>[4x]HHHHHHSSGLVPRGSHMLRRTSSTFSAKRVFVVGGHITTFVGKGSPLFIDKKHPDFGKKENKTLEELLAESINGALQNTGLHDGRAALVDKLVVGNFLGELFSSQGHLGPAAVGSLSGSNSSAFLNKPAVRVEGACASGGLAVQSAWEALLAGTSQIA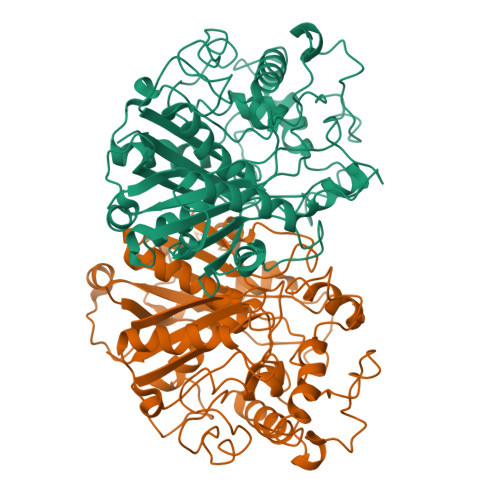LAVGVEVQTTVSARVGGDYLARAAHYKRQRQLDDFTFPCLFARRMKAIQEAGHFTMEDAAYVAAKAYASGNRNPLAHMHARKVTLDFCTQASDKNPNFLGNEIYKPFLRTTDCSQVSDGGAAVILASEEGLQKLGLSPNDNRLVEIKSLASAAGNLYEDSPDLTRMTTSMVAARTALSMAGVKPEQLQVAEVHDAFTIAELLMYEALGIAEYGGAGALIRSGATALDGRIPVNTGGGLLSFGHPVGATGVKQVLEVYRQMKGQCGEYQMKNIPGIGATLNMGGDDKTAVSMVLTNI> GPQKAIIRVIPLKMDPTGKLNLTLEGVFAGVAEITPAE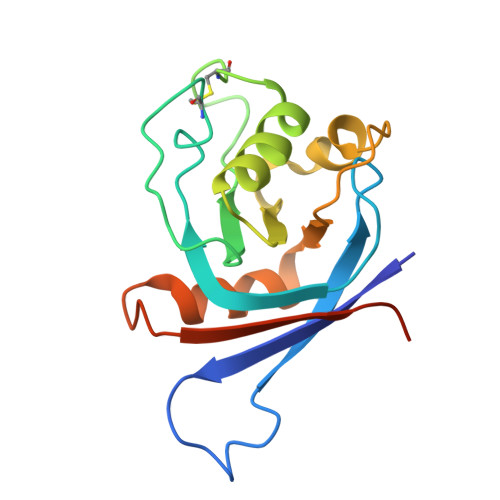GKLMQSHPLYLCNASDDDNLEPGFISIVKLESPRRAPRPCLSLASKARMAGERGASAVLFDITEDRAAAEQLQQPLGLTWPVVLIWGNDAEKLMEFVYKNQKAHVRIELKEPPAWPDYDAAA> GSHMNTEVSSEIYQWVRDELKRAGISQA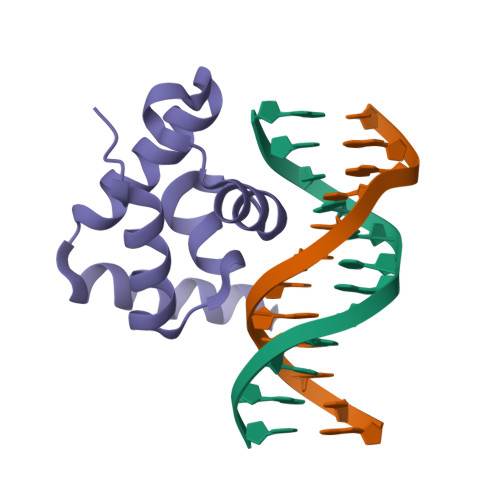VFARVAFNRTQGLLSEILRKEEDPKTASQSLLVNLRAMQNFLQLPEAERDRIYQDERERSLRKRK> SSQIRQNYSTEVEAAVNRLVNLYLRASYTYLSLGFYFDRDDVALEGVCHFFRELAEEKREGAERLLKMQNQRGGRALFQDLQKPSQDEWGTTLDAMKAAIVLEKSLNQALLDLHALGSAQADPHLCDFLESHFLDEEVKLIKKMGDHLTNIQRLVGSQAGLGEYLFECCTLKHD

Ferritin is a self-assembly protein cage consisting of 24 subunits with an 8 nm interior cavity. The 4-fold channel is composed of four E-helices forming a parallel four-helix bundle with C4 symmetry. Herein, we have engineered and constructed a gold clustering site at the 4-fold symmetric axis channel of the apo-ferritin cage. Using a series of X-ray crystal structures, we evaluated the stepwise accumulation process of Au ions into the cage and the formation of a multinuclear Au cluster in our designed cavity.

Our preliminary experiments with gold ions using Cys mutants (161 C/165 C and 168 C/169 C) demonstrate the potential of the 4-fold channel of apo-ferritin as a site for constructing Au clustering. Another important insight is that the side chain of cysteine is relatively short, making the interaction between Au atoms bound on different monomers rather difficult. In addition, the binding mode presents less diversity with a common pattern of one cysteine binding to two Au atoms acting as a bridge. Therefore, to create an Au clustering site at the 4-fold channel, coordination residues with longer side chain and larger rotamer space are needed to build the interaction between Au atoms from different monomers.>[6x]GAMEMRLEKDRFSVNLDVKHFSPEELKVKVLGDVIEVHGKHEERQD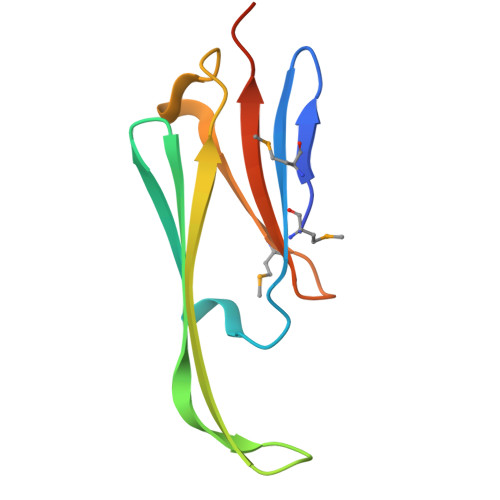EHGFISREFHRKYRIPADVDPLTITSSMSSDGVLTVNGPRKQVSGPER4-(1H-pyrrol-1-yl)aniline | 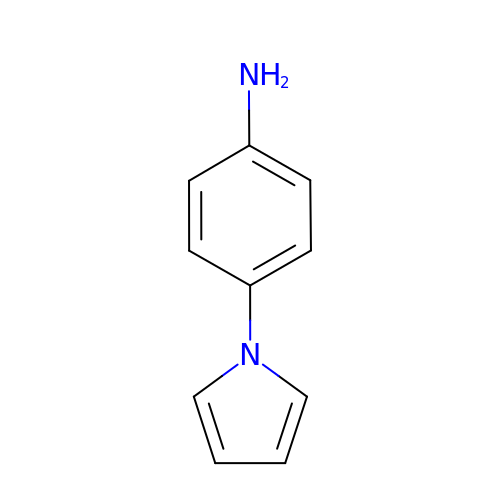C10 H10 N2 | NHLHWHRXMZZWGA-UHFFFAOYSA-N L-NEOPTERIN | C9 H11 N5 O4 | 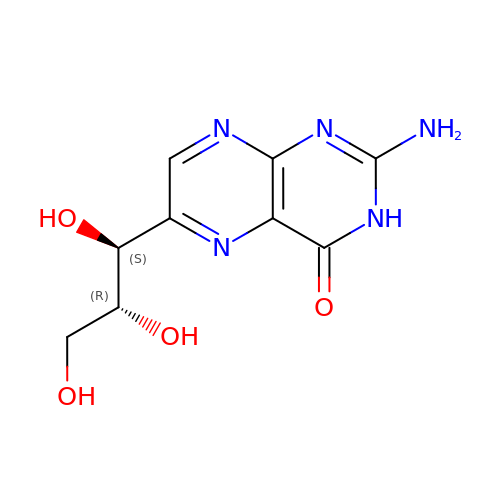BMQYVXCPAOLZOK-XINAWCOVSA-N>MEQNRFKKETKTCSASWPRAPQSTLCATDRLELTYDVYTSAERQRRSRTATRLNLVFLHGSGMS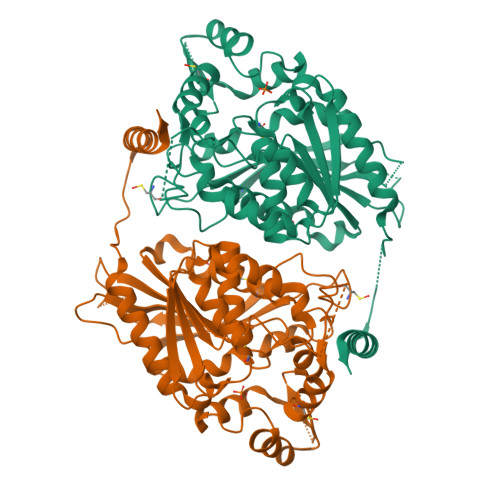KVVWEYYLPRLVAADAEGNYAIDKVLLIDQVNHGDSAVRNRGRLGTNFNWIDGARDVLKIATCELGSIDSHPALNVVIGHSMGGFQALACDVLQPNLFHLLILIEPVVITRKAIGAGRPGLPPDSPQIPENLYNSLRLKTCDHFANESEYVKYMRNGSFFTNAHSQILQNIIDFERTKASGDDEDGGPVRTKMEQAQNLLCYMNMQTFAPFLISNVKFVRKRTIHIVGARSNWCPPQNQLFLQKTLQNYHLDVIPGGSHLVNVEAPDLVIERINHHIHEFVLTSPLQSSHIPQLTLEERAVMFDRAFDSFKNEALVKTTKQKLAAALEHHHHHH[3x]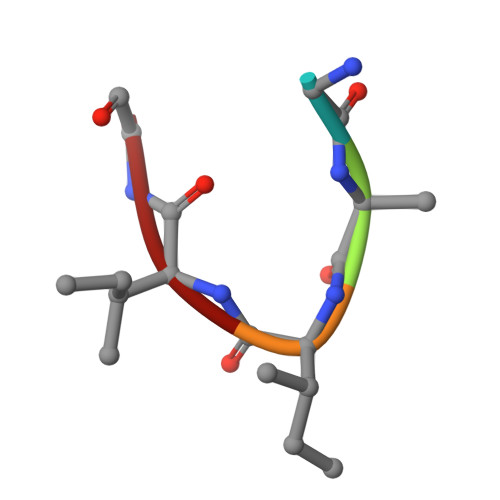> GAIIG> MMAGKSSLFKIILLGDGGVGKSSLMNRYVTNKFDSQ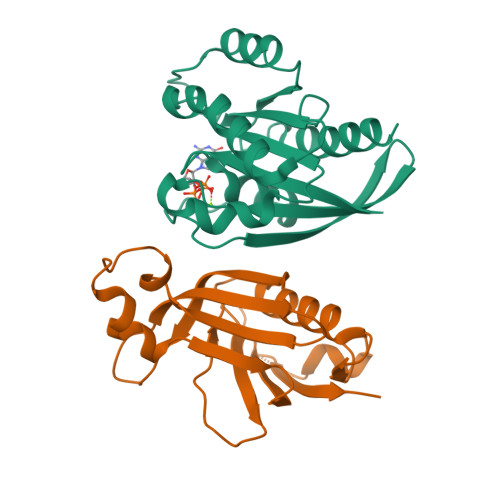LFHTIGVEFLNKDLEVDGHFVTMQIWDTAGLERFRSLRTPFYRGSDCCLLTFSVDDSQSFQNLSNWKKEFIYYADVKEPESFPFVILGNKTDIKERQVSTEEAQAWCKDNGDYPYFETSAKDSTNVAAAFEEAVRRILATEDRSEHLIQTDTVNLHRKPKPNSSLEHHHHHH;> MAHHHHHHATLLYGKNNVLVQPRDDMEAVPGYLSLHQTADVMTLKWTPNQLMNGSVGDLDYEKSVYWDYAVTIRLEEIVYLHCHQQVDSGGTVVLVSQDGIQRPPFRFPKGGHLLQFLSCLENGLLPHGQLDPPLWSQRGKGKVFPKLRKRSPQGSSESTSSDKEDDEATDYVFRIIYPG> MLESKLKAPVFTARTQGRHYGEFVLEPLERGFGVTLGNPLRRILLSSIPGTAVTSVYIEDVLHEFSTIPGVKEDVVEIILNLKELVVRFLDPKMASTTLILRAEGPKEVRAGDFTPSADVEIMNPDLHIATLEEGGKLYMEVRVDRGVGYVPAERHGIKDRINAIPVDAIFSPVRRVAFQVEDTRLGQRTDLDKLTLRIWTDGSVTPLEALNQAVAILKEHLNYFANPEASLLPTPEVSKGEKR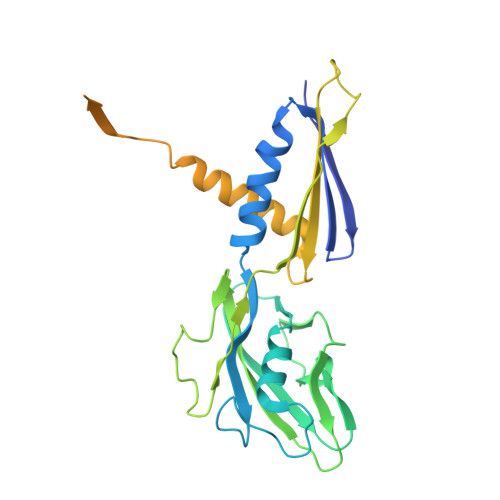ESAEEDLDLPLEELGLSTRVLHSLKEEGIESVRALLALNLKDLRNIPGIGERSLEEIRQALAKKGFTLKE> GSSEVIIDFSTFENRLLALRDRFPSFDGSPSSLVFILGSADEENPYQKTTILHNWLLGYEFPTTLIAVFKEGCVVITSAAKTRYLEEGVAQMNKKLENTFKIELWQSSKEPGHNLKLFEDLVERVREAGSAVGLATKDSYQGKFITEWKGVWDTAVEKHGLNGVDVSLGLSSLWAVKDEKEQAYLQVSSRGSDKFMNLLSDELVRAVDEEIKITDAKLSDNVENEIDKSRFLKKLSPELTPLCPKGEKFDVNYLDWAY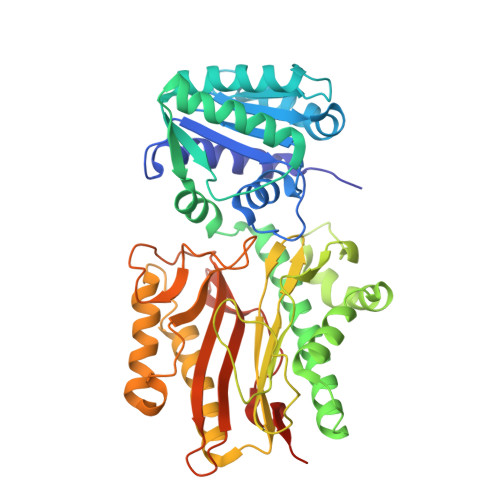SPIIQSGPKYDLRVSARSSETQLDGNGCILASCGIRYKNYCSNISRTFLIDPSDEMTDNYDFLLLLQEEIINNLLRVGATPKQIYDGAVNYINSKKPELSAGFTKNVGSLMGLEFRDSQFVLNNKNDYRKVENGDCFNISLGFNNLKDSKTGASYALQLADTVQLTSGGPKVLTNYTKSRSQISFYFNNEDDGTTKVKSEESK>[5x]GPMAEKLNFEELNSMQRYSQFAVFRAIPGALGSDRAEIVAQAQSFFDGLETAGKVEVRGIYDLAG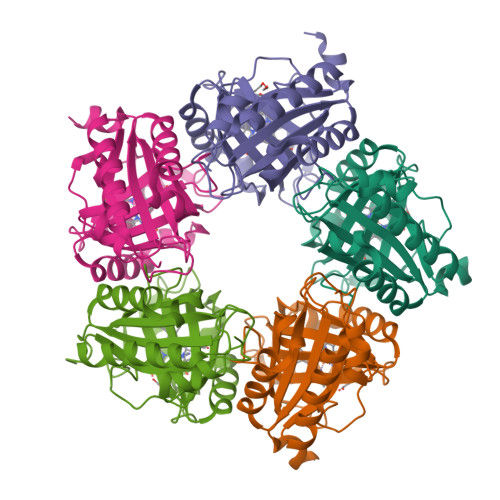CRAEADFMIWWIAEEFEEIQAAFARFRRETVLGQVSEVAWLGNSLHRPAEFNRSHLPSFIMGEIPGDWITVAPFVRSYDWYIMDPQKRRKILAEHGQAARDFPDVRANTVPAFALGDYEWMLAFEAPRLDRIVDLMHKMRYTEARLHVREETPFFTGRRVSEVSELVNVLPG> AMDMTFRYRGPSPKGDQPKAIAGLVEALRDGERFVTLLGATGTGKTVTMAKVIEALGRPALVLAPNKI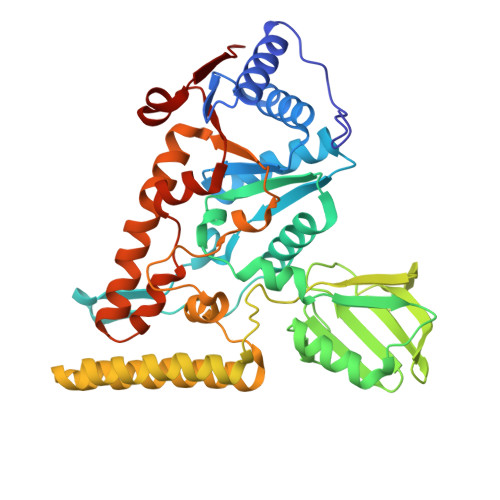LAAQLAAEFRELFPENAVEYFISYYDYYQPEAYVPGKDLYIEKDASINPEIERLRHSTTRSLLTRRDVIVVASVSAIYGLGDPREYRARNLVVERGKPYPREVLLERLLELGYQRNDIDLSPGRFRAKGEVLEIFPAYETEPIRVELFGDEVERISQVHPVTGERLRELPGFVLFPATHYLSPEGLEEILKEIEKELWERVRYFEERGEVLYAQRLKERTLYDLEMLRVMGTCPGVENYARYFTGKAPGEPPYTLLDYFPEDFLVFLDESHVTVPQLQGMYRGDYARKKTLVDYGFRLPSALDNRPLRFEEFLERVSQVVFVSATPGPFELAHSGRVVEQIIR> MGHHHHHHSHVAQFPTPFGGSLDTWAITVEERAKHDQQFHSLKPISGFIT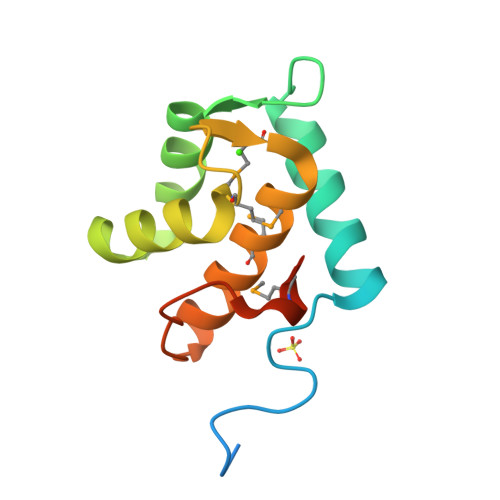GDQARNFFFQSGLPQPVLAQIWALADMNNDGRMDQVEFSIAMKLIKLKLQGYQLPSALPPVMKQQPVAISS> MGKYDGSKLRIGILHARWNAEIILALVLGALKRLQEFGVKRENIIIETVPGSFELPYGSKLFVEKQKRLGKPLDAIIPIGVLIKGSTMHFEYICDSTTHQLMKLNFELGIPVIFGVLTCLTDEQAEARAGLIEGKMHNHGEDWGAAAVEMATKFN;> MEEAELAYLLGELAYKLGEYRIAIRAYRIALKRDPNNAEAWYNLGNAYYKQGRYR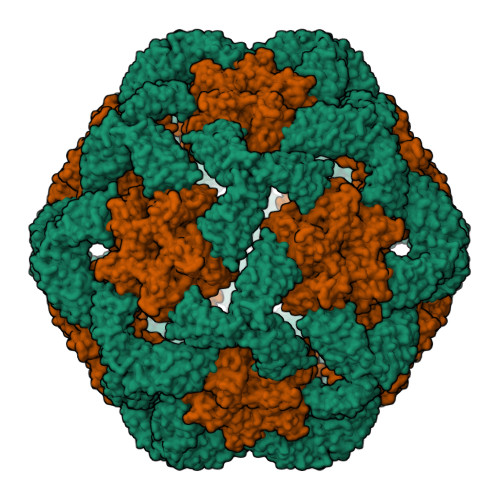EAIEYYQKALELDPNNAEAWYNLGNAYYERGEYEEAIEYYRKALRLDPNNADAMQNLLNAKMREELEHHHHHH> QPQFNEDTLQQRLQALIESAGENWTYAIFWQISHDFDSSTGDNTVILG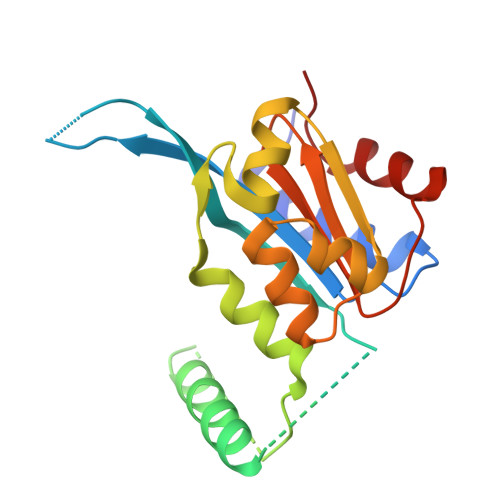WGDGYYKGEEDKEKKKNNTNTAEQEHRKRVIRELNSLISGGIGVSDESNDEEVTDTEWFFLVSMTQSFVNGVGLPGESFLNSRVIWLSGSGALTGSGCERAGQGQIYGLKTMVCIATQNGVVELGSSEVISQSSDLMHKVNNLFNFN> 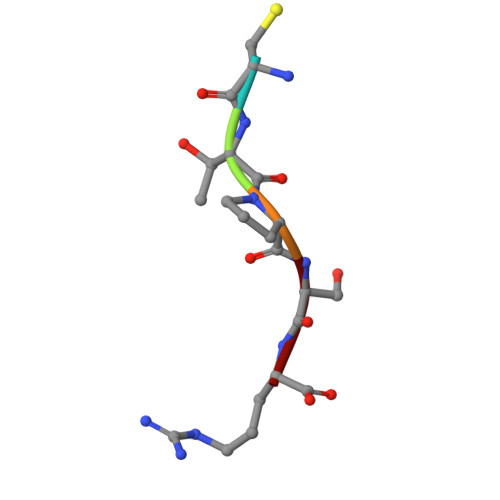CTPSR>[4x]GAMGNHKAALTKQVFTFASELYAYGVREVVISPGSRSTPLALAFEAHPNIKTWIHPDERSAAFFAVGLIKGSERPVAILCTSGTAAANYTPAIAESQISRIPLIVLTSDRPHELRSVGAPQAINQVNMFNNYVSYEFDMPIADDSKETINAIYYQMQIASQYLYGPHKGPIHFNLPFRDPLTPDLNATELLTSEMKILPHYQKSIDASALRHILNKKKGLIIVGDMQHQEVDQILTYSTIYDLPILADPLSHLRKFDHPNVICTYDLLFRSGLDLNVDFVIRVGKPVISKKLNQWLKKTDAFQILVQNNDKIDVFPIAPDISYEISANDFFRSLMEDTTINRVSWLEKWQCLEKKGRKEIKCYLEQATDESAFVGELIKKTSEKDALFISNSMPIRDVDNLLLNKNIDVYANRGANGIDGIVSTALGMAVHKRITLLIGDLSFYHDMNGLLMSKLNNIQMNIVLLNNDGGGIFSYLPQKESATDYFERLFGTPTGLDFEYTAKLYQFDFKRFNSVSEFKNATLLSETSTIYELITNREDNFKQHQILYQKLSEMIHDTL

MenD is a thiamine diphosphate (ThDP)-dependent enzyme that catalyses the conversion of oxoglutarate and isochorismate to 2-succinyl-5-enolpyruvyl-6-hydroxy-3-cyclohexene-1-carboxylic acid (SEPHCHC). Catalysis occurs through two covalent ThDP intermediates as the substrates oxoglutarate and isochorismate are successively added to ThDP before SEPHCHC is released. Sau is an important human pathogen, and uses MK (predominantly MK-8) for both aerobic and anaerobic respiration. In this work, we report that the Sau-MenD is allosterically inhibited by DHNA.

The Sau-MenDIS1 tetramer structure is typical of all known MenD structures to date and, like the Bs-MenD and Ec-MenD structures, is symmetrical, with nearly identical conformations for each monomer (r.m.s.d. using SSM of 0.29–0.44 Å over the length of the chain), and well-defined ThDP and Ca2+ cofactors bound to all four active sites. The three-domain α/β monomeric fold is typical of enzymes from the decarboxylase superfamily of ThDP-dependent enzymes, with domain I (PYR domain, residues 1–200) pairing with domain III (PP domain, residues 364–557) from the other monomer in the dimer to form each of the four paired MenD active sites. The ThDP diphosphate and associated Ca2+ are anchored to the enzyme via domain III (Ser390, Met391, Ser440, Asp438, Gly's 467–469, Asn465, Ile471), as is the ThDP thiazole ring, which is sandwiched between the side chains of Phe471 and Ile416, facilitating the catalytically active V-shaped ThDP conformation. The ThDP aminopyrimidine ring inserts into a pocket between domain I and domain III, forming hydrogen bonds with Asn414, Ile416 and Glu56—the latter playing an important role in proton transfer and stabilization of the various catalytically important aminopyrimidine ring tautomers. There is limited conservation of the allosteric region; we identified only one of three key arginines of the Mtb-MenD arginine cage (Arg97) conserved in Sau-MenD (Arg98), with the other two (Mtb-MenD Arg277 and Arg303) being conservatively replaced by Lys283 and Lys309, respectively. Therefore, structural comparisons of the Sau-MenD structure and DHNA-bound Mtb-MenD were used to gain insight into the structural conservation at the putative allosteric site. These overlays reveal that the likely structural equivalents for the arginine cage are Arg98, Lys283 and Lys309. None of these residues matches the side chain conformers that would be needed for DHNA binding, suggesting that for DHNA to bind, conformational rearrangements would be needed along with backbone movements around the 305–312 region. Mutation of the three Sau-MenD allosteric cage candidates validated a significant role for two (Arg98 and Lys283) in the inhibition of SEPHCHC synthase activity by DHNA.>[4x]MGILDNKVALVTGAGSGIGLAVAHSYAKEGAKVIVSDINEDHGNKAVEDIKAQGGEASFVKADTSNPEEVEALVKRTVEIYGRLDIACNNAGIGGEQALAGDYGLDSWRKVLS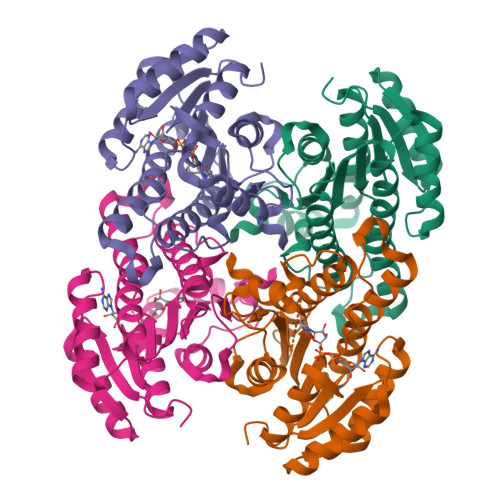INLDGVFYGCKYELEQMEKNGGGVIVNMASIHGIVAAPLSSAYTSAKHAVVGLTKNIGAEYGQKNIRCNAVGPAYIETPLLESLTKEMKEALISKHPMGRLGKPEEVAELVLFLSSEKSSFMTGGYYLVDGGYTAV> MGMWASLDALWEMPAEKRIFGAVLLFSWTVYLWETFLAQRQRRIYKTTTHVPPELGQIMDSETFEKSRLYQLDKSTFSFWSGLYSETEGTLILLFGGIPYLWRLSGRFCGYAGFGPEYEITQSLVFLLLATLFSALAGLPWSLYNTFVI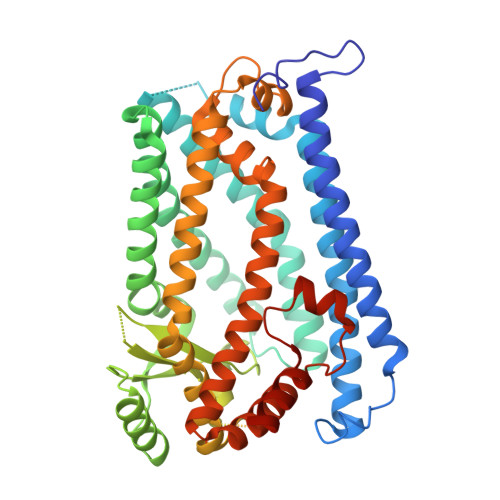EEKHGFNQQTLGFFMKDAIKKFVVTQCILLPVSSLLLYIIKIGGDYFFIYAWLFTLVVSLVLVTIYADYIAPLFDKFTPLPEGKLKEEIEVMAKSIDFPLTKVYVVEGSKRSSHSNAYFYGFFKNKRIVLFDTLLEEYSVLNKDIQEDSGMEPRNEEEGNSEEIKAKVKNKKQGCKNEEVLAVLGHALGHWKLGHTVKNIIISQMNSFLCFFLFAVLIGRKELFAAFGFYDSQPTLIGLLIIFQFIFSPYNEVLSFCLTVLSRRFEFQADAFAKKLGKAKDLYSALIKLNKDNLGFPVSDWLFSMWHYSHPPLLERLQALKTMKQHAENLYFQ>[6x]MPTLPKAEAKELSAFVQSCVEYKTNVCFTDVAAYESNQKGVLSSGLAVLVGTHKQLRDPAVQRLPFYNPAVAEAIERVKEGGTYGVLVEGLANAAGSKFVRVVVGEVPTKASRNNCPARPDVVTALVTAALDEVKEPNTTVDVFVLSNAVLPIAAAVARCGKHNFSAKDGAAAAAYNSGKVSRLQVVFPEPPAIPPKDLEAVATSTQLCQRLVDAPPNLLTTATFTEIAQGYAKALGFDVDVICGDDLCERGYGGIYSVGKAAFEAPRL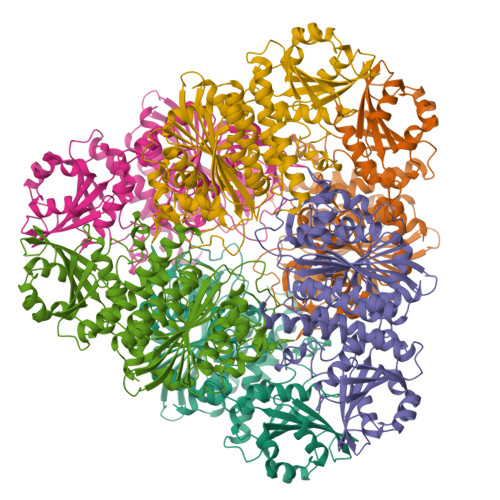VTLLYTPKGTPVKKVSLVGKGIVYDCGGLALKPADYMKLMKHDMGGAAAVFCGFLTAVRLQQPVQLSCTLCLAENAIGPKSYRNDDIIVMKSGKTVEVINTDAEGRIVLGDGVFHATNELSFTPDVVIDMATLTGAQGIATGRHHAGLYVNEEGAEAAMLRAGRESGETCFPVLYCPEYHEPEFKSNHADMTNLMERRDNAGVSCAGYFITTHLSPKFTGAHIHVDLAYPVFNSNGATGFGPALLTEYFRKL>MRPETIPGISLNEDNSHYFYTRAGRRLSAEEVDSWVDQYAGTQVKELMLCPNCMRTSYASQVWDPIWRGYDPAGPDDQPLLASLPPEERVAARGWIHTAWQLHQDGIDIYARWIRRCRQRGISPWISMRMNDVHYVNDERCFLHSEFWRENPQLRRVPYRFAEWTDRAFDYGRAEVREHHLKLIRELAARYDFDGLELDWMRFGFHFRPGYEAEGAEILTAFTAEVRRLLDDWEKRRGHKIHLGARIPSRPATALGLGMDAVTWARRGLVDMLVITPFWASAETDMPVEIWRQLLEGTGVTLAAGLEVLLRPYPDSPLFQTNSLETVRGAAASLLDRGAQRIYLFNYMDSQTAMEDLENYPTLLREIGSLETLAGKPRRHVLTFADTWAPGEPRAIPLPATCRPGEWRAFRLHTGPKPEPGEVIAALGIEGGVAIGPETLEVRVNGELCAFLGLVDLSKPRPDFPVYGFSVPLAAMRRGYNLIEVTARQELRFGWAEFLIRPWHSHHHHHH[2x]

Here we describe the 3-D structure and catalytic center of the defining member, EnvSia156, of this sialidase family. We show, through ligand complexes with products and sialidase inhibitors, that the 3-D structure and active center are indeed an unusual arrangement, with family-conserved histidine and aspartate residues defining the catalytic mechanism that acts with inversion of anomeric configuration; facets not previously observed in the canon of literature for sialidases. The catalytic domain (residues 6–376) comprises a complete (β/α)8-barrel fold while the C-terminal domain (residues 377–502) consists of an eight-stranded β-sandwich. Here we show that GH156 sialidases define a distinct paradigm for sialidase action with His and Asp acting as Brønsted acid and base, respectively, in an inverting mechanism that is unique amongst all exo-sialidases described to date.

To explore the 3-D structure and molecular determinants supporting the unique catalytic mechanism described by Chuzel et al. 26, the structure of EnvSia156 was determined on its own and in complex with N-acetylneuraminic acid (Neu5Ac), N-glycolylneuraminic acid (Neu5Gc), 2-keto-3-deoxy-d-glycero-d-galacto-nononic acid (KDN), and the inhibitor DANA. The absence of related 3-D structures dictated the need for a selenomethionine approach to phasing, so a selenomethionine derivative was crystallized and data collected at three different wavelengths (selenium peak, inflection, and high-energy remote). The resulting refined SeMet structure was subsequently used as the starting model for refinement of unliganded EnvSia156 and complexes with 20 mM Neu5Ac, Neu5Gc, DANA, KDN. Two copies of the protein were present in the asymmetric unit, each composed of two distinct domains. The two copies appear to be related by non-crystallographic symmetry resulting in a dimer, discussed below in light of the interface analysis and SEC-MALLS results. By coloring the structure according to homology, using the same color scheme as in the alignment, it is possible to identify a highly conserved pocket on the “N-terminal” face of the (β/α)8-barrel that sits at both ends of the continuous groove formed by the dimer. Considering its position and conservation, this site is a likely candidate to represent the EnvSia156 catalytic center. The identified conserved pocket indeed shows the presence of three 100% conserved arginines (Arg129, Arg 202, and Arg246), hinting at a sialoside-binding region, although one of them, Arg246, seems to be too buried to be able to interact with the carboxylate moiety of sialic acid. EnvSia156 also displays several highly conserved hydrophobic residues forming a pocket that could potentially accommodate the aglycone moiety of the sialoside substrates.>[2x]PPYTVVYFPVRGRCAALRMLLADQGQSWKEEVVTVETWQEGSLKASCLYGQLPKFQDGDLTLYQSNTILRHLGRTLGLYGKDQQEAALVDMVNDGVEDLRCKYISLIYTNYEAGKDDYV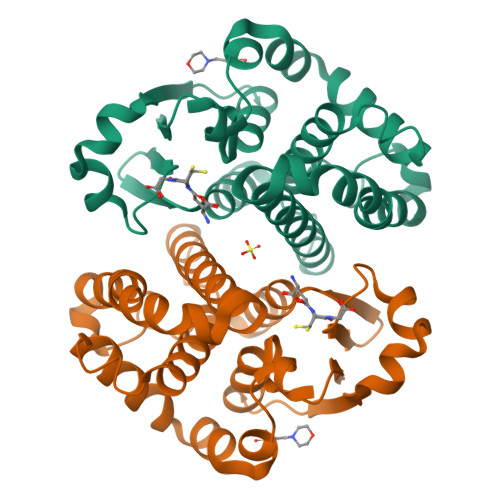KALPGQLKPFETLLSQNQGGKTFIVGDQISFADYNLLDLLLIHEVLAPGCLDAFPLLSAYVGRLSARPKLKAFLASPEYVNLPMDEKSL> MSNDIL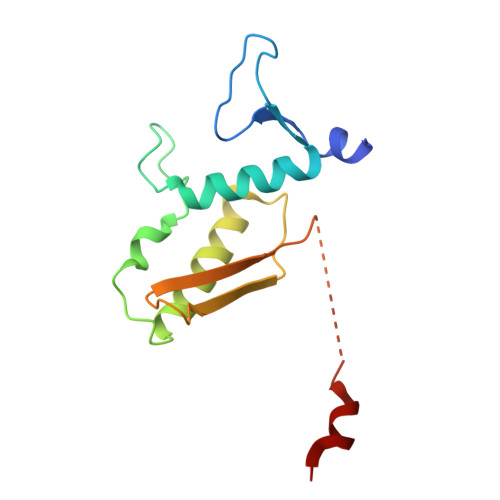KATLGQCWAFPPRFSPDTGVSLTAGVEAVMQSLRVLFMTEPGERIMRESYGGGMHDFIFENITDELLANIHNRIEESILRHEPRALLKDVIIQPDKQEASRLRAQITVYLAGSDLVETVDGTLNIHDGQTLRLL>[2x]DMDLDSYQIALEEVLTWLLSAEDTFQEQDDISDDVEDVKEQF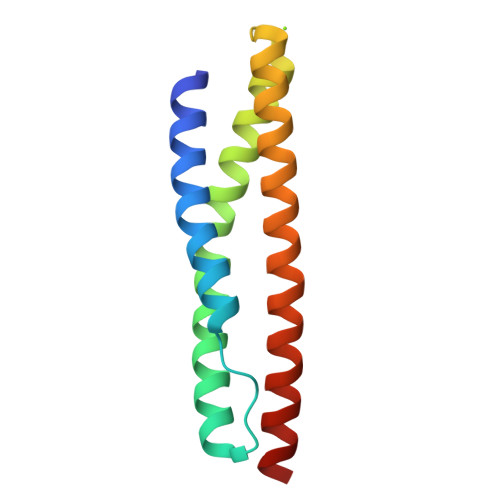ATHETFMMELSAHQSSVGSVLQAGNQLMTQGTLSDEEEFEIQEQMTLLNARWEALRVESMERQSRLHDALMELQKK> LPLQPSSTMGQVGRQLAIIGDDIN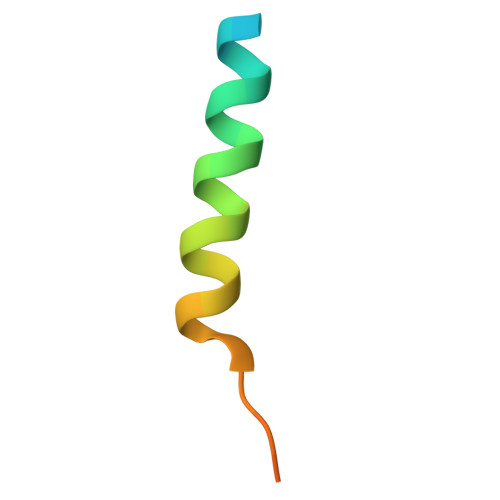RRYDSEFQTM>[2x]NEQRMGRKLAATTLKQCLAKGGARTAFPGTSEYSTARLAYNLRERYAPSAFVFPTTVAQVQNAVFCAKQVGVGIVPRGGGHSYEDYSLGGRDGVLVVDMEGFKQFSYNKAAKTAVVGAGFRLGPLYLALWNAGKVTIPAGNCPTVGIAGHALGGGWGFSSRKFGLVTDNILEVQLVAANGTVVTA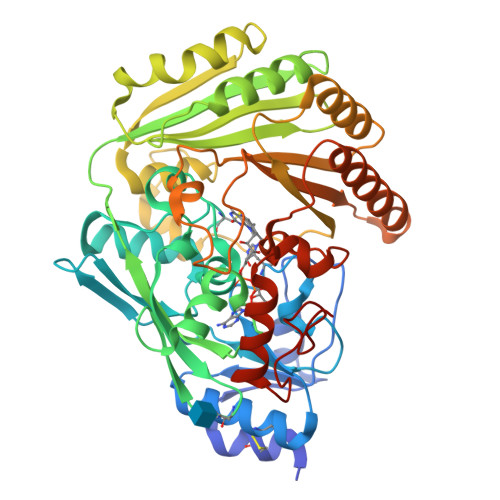NAQKNKDLYFAIRGAGATSYGIVTQFTFRVHDVSAPVTHFKYRWNDKAVLFKNFKSFQSWGLNVPAEISAAFYMDPSGVSWLEGTYLGKKTSLLPLVKTFLASAAPNPTRVEEELNWIQLILVNWNYPSNTNPNQLNNVPFTTNTFKAKSIYVNGPGLSDAGINAMINAMNTGSNAYFIYNLYGSQSAINKVVPGETAFIHRNSLYSIQMVASWSNDNNAVTQTSYITRYWKVVRTYATGQAYQNYIDRDMPLSAYYGSSLSTLIAGKKKWDPQNVFNFPQSIPLKHHHHHHHH(2S)-2-({4-[({(6R)-2,4-diamino-5-[(1-{(2R,4S,5R)-4-hydroxy-5-[(phosphonooxy)methyl]tetrahydrofuran-2-yl}-2,4-dioxo-1,2,3,4-tetrahydropyrimidin-5-yl)methyl]-5,6,7,8-tetrahydropyrido[3,2-d]pyrimidin-6-yl}methyl)amino]benzoyl}amino)pentanedioic 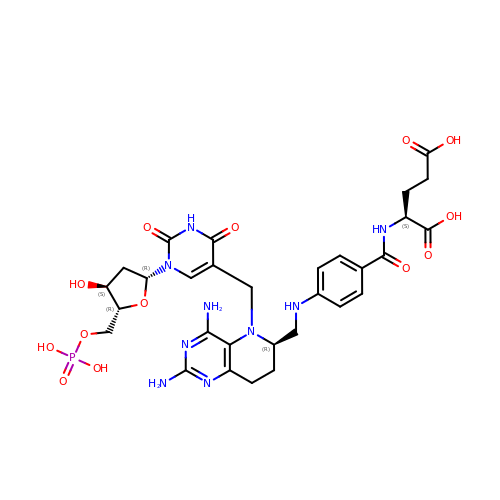acid (non-preferred name) | C30 H38 N9 O13 P | OYTZJQBUPHBEFY-WHCFWRGISA-N>[2x]GPHMDLASLRAQQIELASSVIR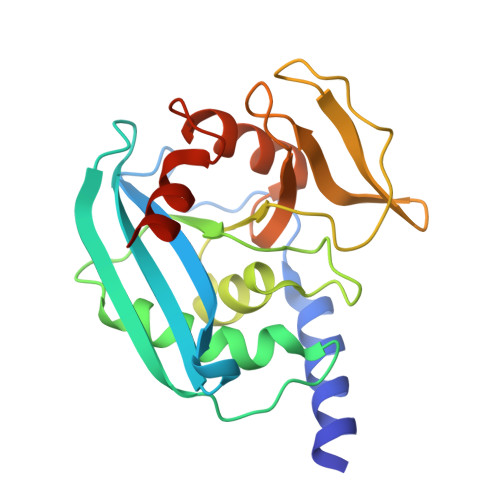EDRLDKDPPDLIAGADVGFEQGGEVTRAAMVLLKYPSLELVEYKVARIATTMPYIPGFLSFREYPALLAAWEMLSQKPDLVFVDGHGISHPRRLGVASHFGLLVDVPTIGVAKKRLCGKFEPLSSEPGALAPLMDKGEQLAWVWRSKARCNPLFIATGHRVSVDSALAWVQRCMKGYRLPEPTRWADAVASERPA>QAAKQLSQNFLLDLRLTDKIVRKAGNLTNAYVYEVGPGPGGITRSILNADVAELLVVEKDTRFIPGLQMLSDAAPGKLRIVHGDVLTFKVEKAFSESLKRPWEDDPPNVHIIGNLPFSVSTPLIIKWLENISCRDGPFVYGRTQMTLTFQKEVAERLAANTGSKQRSRLSVMAQYLCNVRHIFTIPGQAFVPKPEVDVGV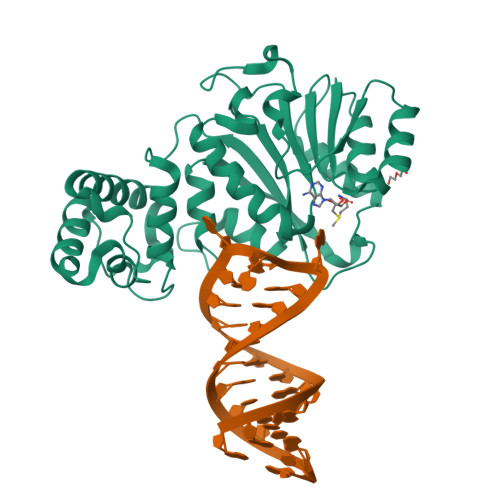VHFTPLIQPKIEQPFKLVEKVVQNVFQFRRKYCHRGLRMLFPEAQRLESTGRLLELADIDPTLRPRQLSISHFKSLCDVYRKMCDEDPQLFAYNFREELKRRKSKNEEKEEDDAENYRL[2x]>[2x]MISLADLQRRIETGELSPNAAIAQSHAAIEAREKEVHAFVRHDKSARAQASGPLRGIAVGIKDIIDTANMPTEMGSEIYRGWQPRSDAPVVMMLKRAGATIIGKTTTTAFASRDPTATLNPHNTGHSPGGSSSGSAAAVGAGM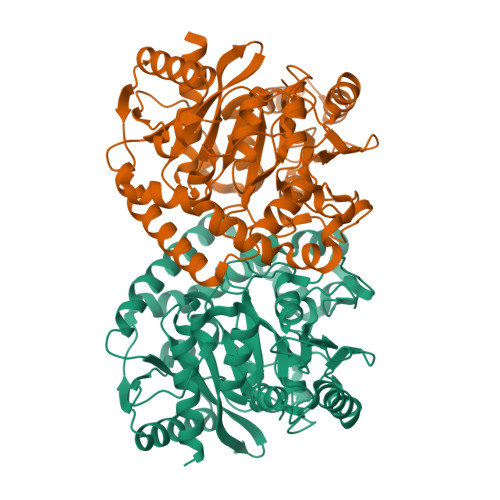IPLALGTQTGGSVIRPAAYCGTAAIKPSFRMLPTVGVKCYSWALDTVGLFGARAEDLARGLLAMTGRSEFSGIVPAKAPRIGVVRQEFAGAVEPAAEQGLQAAIKAAERAGASVQAIDLPEAVHEAWRIHPIIQDFEAHRALAWEFSEHHDEIAPMLRASLDATVGLTPKEYDEARRIGRRGRRELGEVFEGVDVLLTYSAPGTAPAKALASTGDPRYNRLWTLMGNPCVNVPVLKVGGLPIGVQVIARFGNDAHALATAWFLEDALAK>[8x]MGRIKNKQFAVIGLGRFGGSICKELHRMGHEVLAVDINEEKVNAYASYATHAVIANATEENELLSLGIRNFEYVIVAIGPNIQASTLTTLLLKELDIPNIWVKAQNYY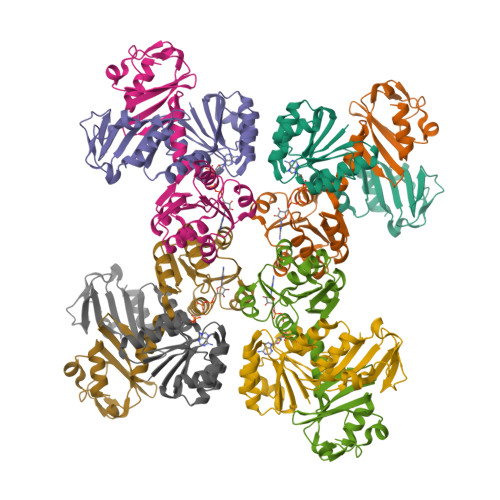HHKVLEKIGADRIIHPEKDMGVKIAQSLSDENVLNYIDLSDEYSIVELLATRKLDSKSIIDLNVRAKYGCTILAIKHHGDICLSPAPEDIIREQDCLVIMGHKKDIKRFENEGM> MASIPSAAPSWRKMQIPRPLQRLFDYFPLRIYEPNELPERSQQLTSGDLPTLYVFSTDSDARLGLPSFNPGCLKWQTLLRLANLDFRILPSTNHSSPTGSLPFLLPPRTSPTASPAPIPASGLLSFARKNPWRPGKAADLDLGHLDADLPPRAQAYLALITHSLRNAWLCALYLDPTHDALLRRLYVDPASSSRAVRAALLHQLRRAAAEQVATASSGGGKIVSLAPVDSADGIDEEAVYRSARDALDALASLLRESETAWFFGTERPGSFDAALFSYTHLMVEYMSEEEDTESAKGRVSLGRMVKEAGNGELAEHRERMLGVAWPEWDGYRR;> MASSLGFGGSNAVDKVNATTTPGTVATPNSGPTKMLDEHILTPASISTLEVHGATNTRRSLLDQIFKPVLEDTAAAGTTLGQVLDRVGAATKKLARFDIFKEEGFGVFLSEAAPPQSAPPTDRTDLDISIRVKEKSRLVFSAGTDFGNAEGSAYTNAVVRNIFGGAETLTVNASTGTRTRSAYNATFSTPINGNPDLRLSVEALRSATQKPWASHEEHLTGANLRLAWLTEKGDTHALAYSSVWRQLTGLAPTASPTVRADAGDSLKSSLTHTFTRDRRDNPMLPQSGYLFRSVSELAGWGPLNGDVSFAKTEVEASGALPVAIPGLAGKSGVSVGGGLRLGVLYPLPLGYSLTGAAQPSRINDRFQLGGPNDVRGFKIGGLGPHDGVDAVGGDVFAAGSVNALLPLPRTGPDSPLRLQLYANAGRLVALNSKGTDKEGKEGLAMDSAAVFKGVKSAVGKLTNGIPSLAAGVGLVYAHPVARFELNFSLPLVLRRGEEGRKGLQVGVGISFL;> MAVQLHVWGPAFGLPSIDAECLAAIAYLAQTLGSADYQLIQSSPSAVPTQHLPTLYDSRTSTWIGGFTSITAHLHTHPPPTFQSAPQPTDGSSSTTTTTTTTTTAASATADGTAYTAFLSAHAAPLLALSLYVSSANYGAATRPAYSAVLPLPLPWTEPPAVRAAMARRAAHLGLSSLDADAAAERARAEERRAAADGWVAVPPHATAGRAAGGGGGGGGGGGKGGGVAAVLTPEQKSRIRLEEAAREVLDVLAEVDWAAGGGGRQVAAEVRCLAFGYLALMLLPDVPRPWLREIMEGRYPALCTFVRDFRARVFPQGGKLLPWADGGAQASASASASASAVALRFVRAVMAEVPLVGEWWSRWWTARKKREVLASKGAKPAPSNDLLLLLGAGLGLTVVGAGVFFYRGLPPFGEAVQVWRKPVVGLSSFGAAGAMFSGALYGLD

The SAM complex facilitates outer membrane β-barrel precursor protein folding and insertion into the outer membrane. The SAM complex consists of one copy each of Sam50, which spans the mitochondrial outer membrane, and Sam35 and Sam37, which sit on the cytosolic side of the membrane. Sam50 forms a 16-stranded β-barrel which is minimally closed between strands β1 and β16. The structures of Sam35 and Sam37 reveal that they each adopt a GST-like fold, which is also completely different from the BAM lipoproteins.

The cryoEM structure of the SAM complex in lipid nanodiscs was reconstructed from 179,509 particles and yielded a 3.4 Å resolution structure. The resolution was sufficient to allow ab initio tracing of a majority of the folds of all three subunits. In lipid nanodiscs, the SAM complex is monomeric and contains one copy each of Sam50, Sam35, and Sam37. Sam50 forms a 16-stranded transmembrane β-barrel with a single POTRA domain extending into the intermembrane space. Sam35 and Sam37 are located on the cytosolic side of the membrane, where Sam35 caps the barrel lumen of Sam50 and also interacts extensively with Sam37. The orientations of Sam35 and Sam37, as well as visualization of the lipid nanodisc, suggest that Sam35 and Sam37 interact peripherally with the outer leaflet of the membrane and residues 339–353 of Sam37 form an amphipathic α-helix that appears to interact with the membrane. In this structure, the highest resolution is observed for the Sam50 β-barrel and for Sam35, with lower resolution (and more flexibility) observed for Sam37 and the Sam50 POTRA domain. When the map is filtered to low resolution, the first of two predicted transmembrane α-helices in Sam37 is visible; however, it is not visible when filtered to high resolution. It appears that the relatively large size of the lipid nanodisc compared to the Sam50 β-barrel prevents optimal particle alignment and further resolution improvement. The reduced resolution in this domain in the lipid nanodisc structure further illustrates its mobility.Following an extensive screen of prokaryotic homologues with high (>40%) amino acid sequence identity to eukaryotic SLC7 transport proteins, we identified a suitable candidate from the thermophilic bacterium Geobacillus Kaustophilus, GkApcT. To address these questions, we determined the crystal structure of a close prokaryotic SLC7 homologue in complex with bound l-alanine and l-arginine ligands and studied its transport mechanism using in vitro biochemical assays. GkApcT was determined to be proton-coupled, with uptake of l-[3H]-Ala observed in the presence of a membrane potential, negative inside and a pH gradient, alkaline inside. Crystal structures of APC superfamily transporters have revealed a conserved ‘5 + 5 inverted topology’ fold, wherein the first five TM helices are related to the second five helices via a pseudo two-fold symmetry axis running parallel to the plane of the membrane.

In particular, Met321, Ala119, Val317 and Ile234 all adopt smaller side chains in the human proteins, being serine, glycine, serine and valine respectively. However, we discovered that Met321Ser was able to recognise and transport both l-Arg and l-Lys to a greater extent than the wild-type protein. Indeed, the affinity of this variant for arginine is significantly increased as demonstrated by a reduction in the IC50 value from 6 mm in the WT to 11.4 μm in the M321S variant. To further validate this result, we obtained a crystal structure at 3.13 Å of the Met321Ser variant with bound l-Arg. The structure shows that replacement of Met321 with serine does not affect the position of the helices within the protein, with a r.m.s.d. of 1.15 Å over 480 Cα atoms when compared to the WT structure. As expected, replacement of Met321 with serine substantially opens up the ligand binding site facilitating the increased size of the l-Arg ligand. The l-Arg is positioned with the α-carboxy and amino termini making identical interactions to those observed with l-Ala, with the side chain extending down into the space opened up by removal of the methionine. In our structure, the guanidinium group sits close to both Glu115 and Asp237. However, the overlay of AdiC and GkApcT suggests that the guanidinium group of arginine will be accommodated in a different position than observed in AdiC, due to TM3 being positioned further into the binding pocket, pushing the side chain towards the conserved serine in the mammalian proteins. The complexes with bound alanine and arginine reveal the molecular basis for amino acid selectivity is based on steric restrains rather than charge complementarity, providing insight into how the SLC7 family has evolved to select specific sub-sets of amino acids.

> MNLFRKKPIQLLMKESGAKGASLRKELGAFDLTMLGIGAIIGTGIFVLTGVAAAEHAGPALVLSFILSGLACVFAALCYAEFASTVPVSGSAYTYSYATFGELIAWILGWDLILEYGVASSAVAVGWSGYFQGLLSGFGIELPKALTSAYDPAKGTFIDLPAIIIVLFITFLLNLGAKKSARFNAVIVAIKVAVVLLFLAVGVWYVKPENWTPFMPYGFSGVATGAATVFFAYIGFDAVSTAAEEVRNPQRDMPIGIIVSLLVCTLLYIAVSLVLTGIVPYEQLNVKNPVAFALNYIHQDWVAGFISLGAIAGITTVLLVSMYGQTRLFYAISRDGLLPKVFARISPTRQVPYVNTWLTGAAVAVFAGIIPLNKLAELTNIGTLFAFITVSIGVLVLRKTQPDLKRAFRVPFVPVVPILAVLFCGYLVLQLPAMTWIGFVSWLLIGLVIYFIYGRKHSELN;> MLGNMNVFMAVLGIILFSGFLAAYFSH>MRTSKKEMILRTAIDYIGEYSLETLSYDSLAEATGLSKSGLIYHFPSR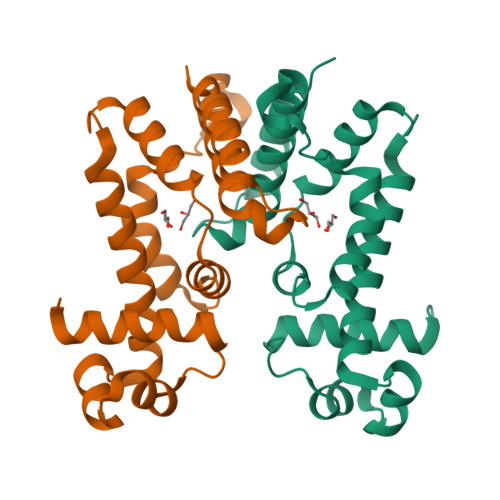HALLLGMHELLADDWDKELRDITRDPEDPLERLRAVVVTLAENVSRPELLLLIDAPSHPDFLNAWRTVNHQWIPDTDDLENDAHKRAVYLVQLAADGLFVHDYIHDDVLSKSKRQAMLETILELIPSQTLEHHHHHH[2x]> GSKRKSEAQENIIKNKDELEDFEQGEKYLTLTVSKNDFKKMEVVGQFNLGFIIVTRKVDNKYDLFIVDQHASDEKYNFETLQAVTVFKSQKLIIPQPVELSVIDELVVLDNLPVFEKNGFKLKIDEEEEFGSRVKLLSLPTSKQTLFDLGDFNELIHLIKEDGGLRRDNIRCSKIRSMFAMRACRSSIMIGKPLNKKTMTRVVHNLSEL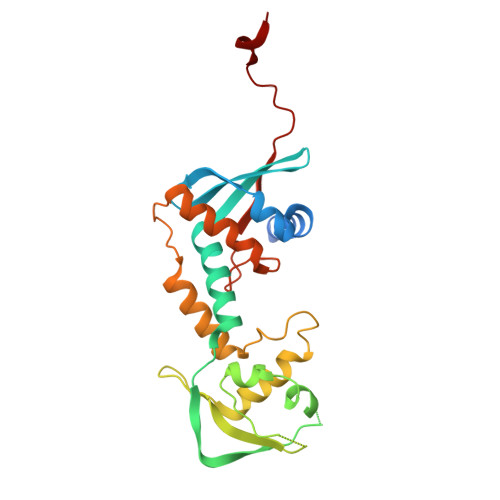DKPWNCPHGRPTMRHLMELRDWSSFSKDYEI>MTLVPDLTATDLARHRWLTDNSWTRPTWTVAELEAAKAGRTISVVLPALNEEETVGGVVETIRPLLGGLVDELIVLDSGSTDD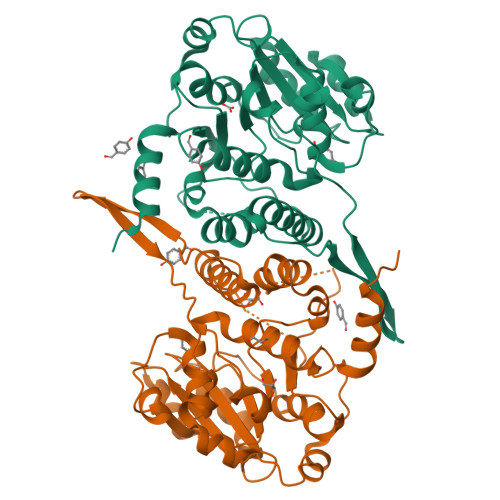TEIRAMAAGARVISREVALPEVAPQPGKGEVLWRSLAATTGDIIVFIDSDLIDPDPMFVPKLVGPLLLSEGVHLVKGFYRRPLKTSGSEDAHGGGRVTELVARPLLAALRPELTCVLQPLGGEYAGTRELLMSVPFAPGYGVEIGLLVDTYDRLGLDAIAQVNLGVRAHRNRPLTDLAAMSRQVIATLFSRCGVPDSGVGLTQFFADGDGFSPRTSEVSLVDRPPMNTLRGKLAAALEHHHHHH[2x]(2S)-2-(5-{[(2-amino-4-oxo-3,4-dihydro[1]benzothieno[2,3-d]pyrimidin-5-yl)methyl]amino}-1-oxo-1,3-dihydro-2H-isoindol-2-yl)pentanedioic 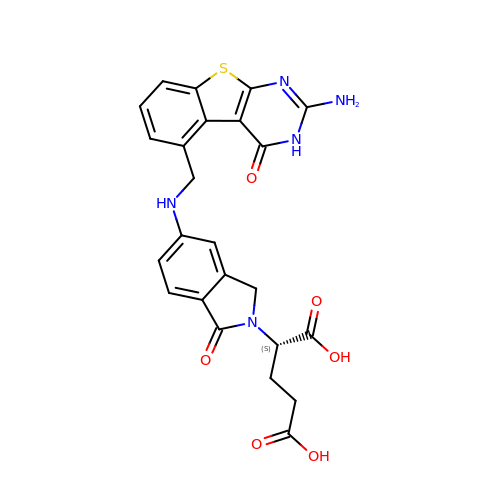acid | C24 H21 N5 O6 S | QPDXRVRRCIFNSL-HNNXBMFYSA-N>[4x]MKIWSKEEVVNKLHEIKNKGYLSVPTDMFRTDDGVVGQILERQFGVQENNITLGDLGEFELKGMRNRKAKSNLTLFHKKPVAGQTVIQIFNRFGYVKPSSRNPEVMKKKLFTTIKGGRLNN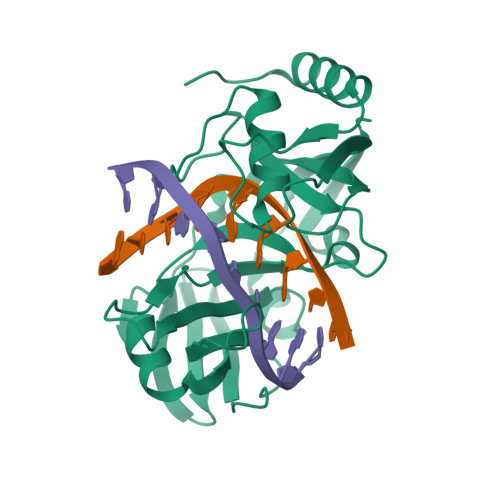LGLTLNAKHASEINLYYQDEYLSTWDLNLSKIEKLVLVFAETIGRANSPEEQFHFTKAYMLTEINDITSLINDGVLVMDLCIDQDLSKSKGPHDRGPHLRIPISKLDKLYRNIERLL>[2x]MGSSHHHHHHSSGENLYFQGHMMEAAASEPSLDLDNLKLLELIGRGRYGAVYKGSLDERPVAVKVFSFANRQNFINEKNIYRVPLMEHDNIARFIVGDERVTADGRMEYLLVMEYYPNGSLCKYLSLHTSDWVSSCRLAHSVTRGLAYLHTELPRGDHYKPAISHRDLNSRNVLVKNDGTCVISDFGLSMRLTGNRLVRPGEEDNAAISEVGTIRYMAPEVLEGAVN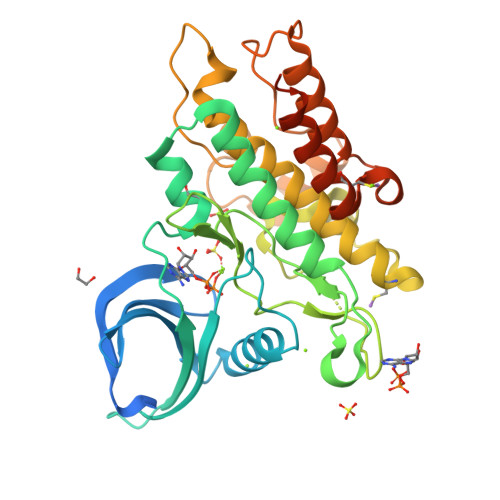LRDCESALKQVDMYALGLIYWEIFMRCTDLFPGESVPEYQMAFQTEVGNHPTFEDMQVLVSREKQRPKFPEAWKENSLAVRSLKETIEDCWGQDAEARLTAQCAEERMAELMMIWERNKSVSPTVNPMSTAMQNER(3S,3aR,4S,6S,6aS,8R,9R,9aR,9bS)-6-(acetyloxy)-4-(butanoyloxy)-3,3a-dihydroxy-3,6,9-trimethyl-2-oxododecahydroazuleno[4,5-b]furan-8-yl (2Z)-2-methylbut-2-enoate | C26 H38 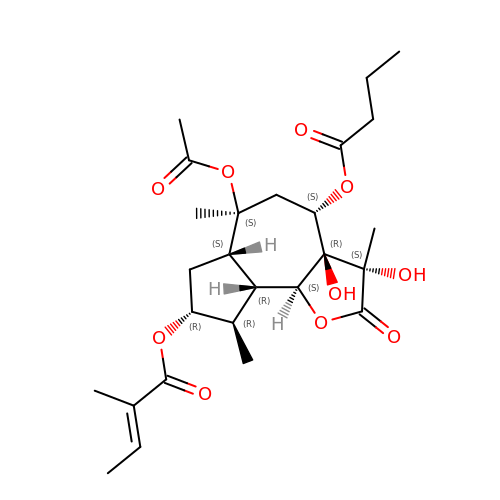O10 | INROUDCDOCKFKL-SBRSFKGSSA-N> MTTAPSLVPVTTPSQHGAGVPHLGIDPFALDYFADPYPEQETLREAGPVVYLDKWNVYGVARYAEVYAVLNDPLTFCSSRGVGLSDFKKEKPWRPPSLILEADPPAHTRTRAVLSKVLSPATMKRLRDGFAAAADAKIDELLARGGNIDAIADLAEAYPLSVFPDAMGLKQEGRENLLPYAGLVFNAFGPPNELRQSAIERSAPHQAYVAEQCQRPNLAPGGFGACIHAFSDTGEITPEEAPLLVRSLLSAGLDTTVNGIAAAVYCLARFPDEFARLRADPSLARNAFEEAVRFESPVQTFFRTTTRDVELAGATIGEGEKVLMFLGSANRDPRRWDDPDRYDIT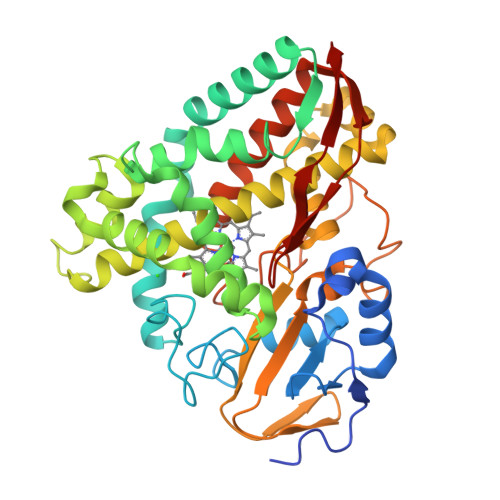RKTSGHVGFGSGVHMCVGQLVARLEGEVVLAALARKVAAIEIAGPLKRRFNNTLRGLESLPIQLTPA> MKHHHHHHMKQNSPLDEENLTQENQDRGTHVDRGLASANVDFAFSLYKQLVLKAPDKNVIFSPVSISTALAFLSLGAHNTTLTEILKGLKFNLTETSEAEIHQSFQHLLRTLNQSSDELQLSMGNAMFVKEQLSLLDRFTEDAKRLYGSEAFATDFQDSAAAKKLINDYVKNGTRGKITDLIKDLDSQTMMVLVNYIFFKAKWEMPFDPQDTHQSRFYLSKKKWVMVPMMSLHHLTIPYFRDEELSCTVVQLNYTGNASVFFILPDQDKMEEVEAMLSRETLARWGDSLEFREIGELYLPKFSISRDYNLNDILLQLGIEEAFTSKADLSGITGARNLAVSQVVHKAVLDVFEEGTEASAATAVKI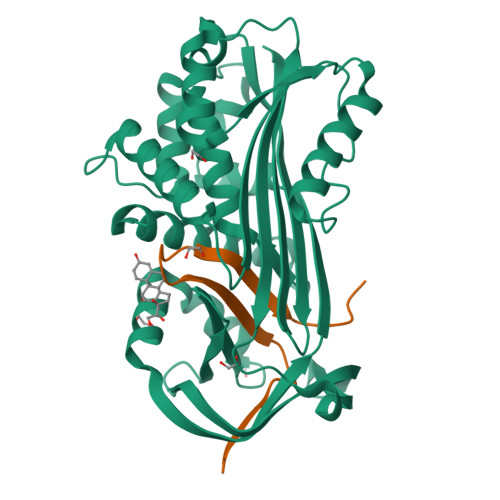TLL;> SALVETRTIVRFNRPFLMIIVDHFTWSIFFMSKVTNPKQA> ATLNRLREPLLRRLSELLDQAPEGRGWRR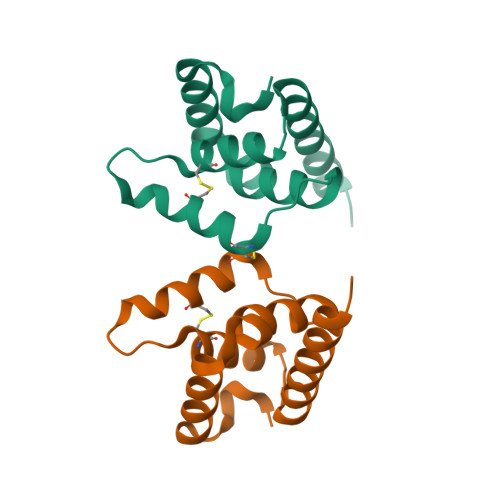LAELAGSRGRLRLSCLDLEQCSLKVLEPEGSPSLCLLKLMGEKGCTVTELSDFLQAMEHTEVLQLLSP> DCPSGWSSYEGNCYKFFQQKMNWADAERFCSEQAKGGHLVSIKIYSKEKDFVGDLVTKNIQSSDLYAWIGLRVENKEKQCSSEWSDGSSVSYENVVERTVKKCFALEKDLGFVLWINLYCAQKNPFVCKSPPP;> DCPPDWSSYEGHCYRFFKEWMHWDDAEEFCTEQQTGAHLVSFQSKEEADFVRSLTSEMLKGDVVWIGLSDVWNKCRFEWTDGMEFDYDDYYLIAEYECVASKPTNNKWWIIPCTRFKNFVCEFQA;> DTPEPPLHNFYCSKLLDLVFLLDGSSMLSEAEFEVLKAFVVGMMERLHISQKRIRVAVVEYHDGSRAYLELKARKRPSELRRITSQIKYTGSQVASTSEVLKYTLFQIFGKIDRPEASHITLLLTASQEPPRMAR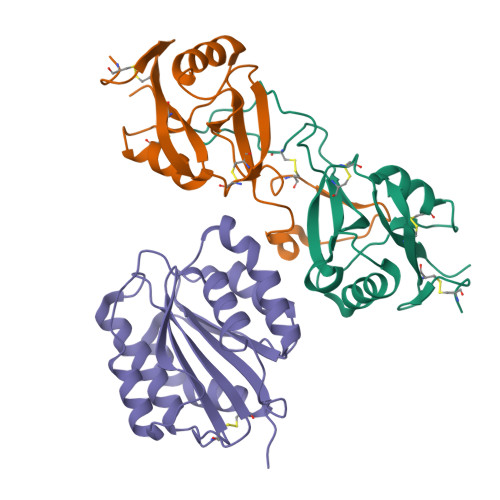NLVRYVQGLKKKKVIVIPVGIGPHASLKQIRLIEKQAPENKAFLLSGVDELEQRRDEIVSYLCDLAPEAPAPT>[2x]ARDISIEDLLARKPKDLDDSAVAAFLKDKVVLVSGAGGTIGSELCKQCIKFGAKHLIMVDHSEYNLYKINDDLNLYKEKITPILLSILDKQ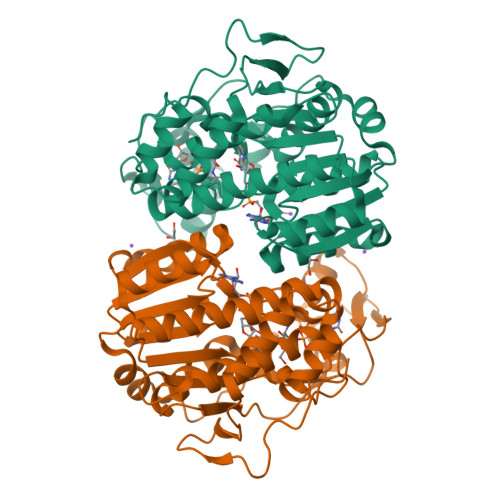SLDEVLKTYKPELILHAAAYKHVPLCEQNPHSAVINNILGTKILCDSAKENKVAKFVMISTNAAVRPTNIMGCTKRVCELYTLSMSDENFEVACVRFGNVLGSSGSVIPKFKAQIANNEPLTLTHPDIVRYFMLVAEAVQLVLQAGAIAKGGELFVLDMGKPVKIIDLAKKMLLLSNRNDLEIKITGLRKGEKLYEELLIDENDAKTQYESIFVAKNEKVDLDWLNKEIENLQICEDISEALLKIVPEFKHNKEGIAAGFNRIPAAALEHHHHHH> ADYDLKFGMNNGTSSNEYKAAEMFAKEVKEKSQGKIEISLYPSSQLGDDRAMLKQLKDGSLDFTFAESARFQLFYPEAAVFALPYVISNYNVAQKALFDTEFGKDLIKKMDKDLGVTLLSQAYNGTRQTTSNRAINSIADMKGLKLRVPNAATNLAYAKYVGASPTPMAFSEVYLALQTNAVDGQENPLAAVQAQKFYEVQKFLAMTNHILNDQLYLVSNETYKELPEDLQKVVKDAAENAAKYHTKLFVDGEKDLVTFFEKQGVKITHPDLVPFKESMKPYYAEFVKQTGQKG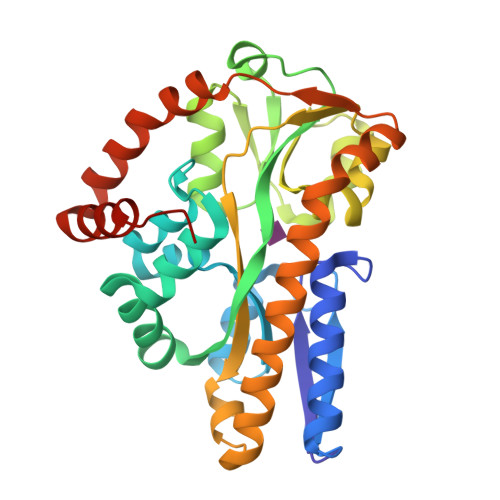ESALKQIEAINPHHHHHH The recently discovered metagenomic-derived polyester hydrolase PHL7 is able to efficiently degrade amorphous polyethylene terephthalate (PET) in post-consumer plastic waste. PHL7 is a thermophilic polyester hydrolase isolated from a plant compost metagenome along with six homologs (PHL1-6). It rapidly hydrolyzes amorphous PET at 70 °C yielding terephthalic acid (TPA) and ethylene glycol (EG), outperforming all previously reported PET-hydrolytic enzymes, including engineered variants. All polyester hydrolases share an α/β-hydrolase structure with a canonical catalytic triad comprised of serine, histidine and aspartate.

We cocrystallized the inactive variant PHL7 S131A along with the PET hydrolysis product TPA. Addition of Ca2+ or Mg2+ improves the thermostability of PHL7 by up to 7 °C4. In a crystal structure of PHL7 that was obtained in the presence of 10 mM Mg2+ ions, we identified a magnesium-binding site comprised of E13, D246 and D247. The Mg2+ ion is complexed by the carboxyl sidechain of D246 and five water molecules in the first interaction shell forming an octahedral geometry. Three of the five water molecules in turn interact with the sidechains of E13, D246, and D247 while the other two are only coordinated by the divalent metal ion. This Mg2+-binding site of PHL7 resembles a Zn2+-binding site identified in the thermophilic homolog Cut190 (binding site 4), which was described as a site unrelated to PET-hydrolytic activity. In summary, two metal binding sites have been identified at the surface of PHL7. Similar to previous studies on other polyester hydrolases, these may as well serve as future mutagenesis targets to increase the thermal stability of PHL7. The two metal binding sites are 26 Å apart and may act independently and thus in an additive manner to increase protein stability.

>[2x]MANPYERGPDPTESSIEAVRGPFAVAQTTVSRLQADGFGGGTIYYPTDTSQGTFGAVAISPGFTAGQESIAWLGPRIASQGFVVITIDTITRLDQPDSRGRQLQAALDHLRTNSVVRNRIDPNRMAVMGHAMGGGGALSAAANNTSLEAAIPLQGWHTRKNWSSVRTPTLVVGAQLDTIAPVSSHSEAFYNSLPSDLDKAYMELRGASHLVSNTPDTTTAKYSIAWLKRFVDDDLRYEQFLCPAPDDFAISEYRSTCPFLEHHHHHH>[2x]GSPFYIKSSPSPQKRYQDTPGVEHIPVVQIDLSVPLKVP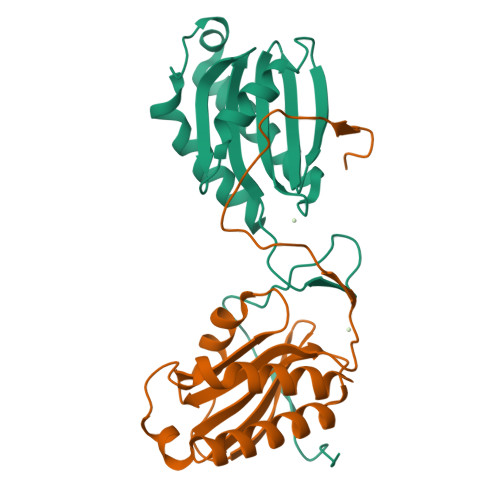GLPMSDQYVKLEEAMAILFAVVARGTTILAKHAWCGGNFLEVTEQILAKIPSENNKLTYSHGNYLFHYICQDRIVYLCITDDDFERSRAFSFLNEVKKRFQTTYGSRAQTALPYAMNSEFSSVLAAQLKHHSEN> MAYPGHPGAGGGYYPGGYGGAPGGPAFPGQTQDPLYGYFAAVAGQD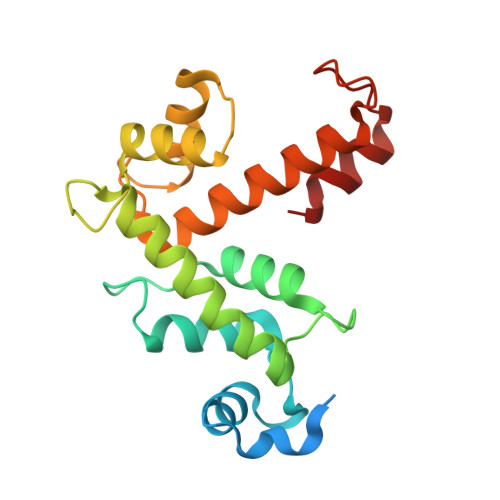GQIDADELQRCLTQSGIAGGYKPFNLETCRLMVSMLDRDMSGTMGFNEFKELWAVLNGWRQHFISFDTDRSGTVDPQELQKALTTMGFRLSPQAVNSIAKRYSTNGKITFDDYIACCVKLRALTDSFRRRDTAQQGVVNFPYDDFIQCVMSV> FSGSEATAAILSRAPWSLQSVNPGLKTNSSKEPKFTKCRSPERETFSCHWTDEVHHGTKNLGPIQLFYTRRNTQEWTQEWKECPDYVSAGENSCYFNSSFTSIWIPYCIKLTSNGGTVDEKCFSVDEIVQPDPPIALNWTLLNVSLTGIHADIQVRWEAPRNADIQKGWMV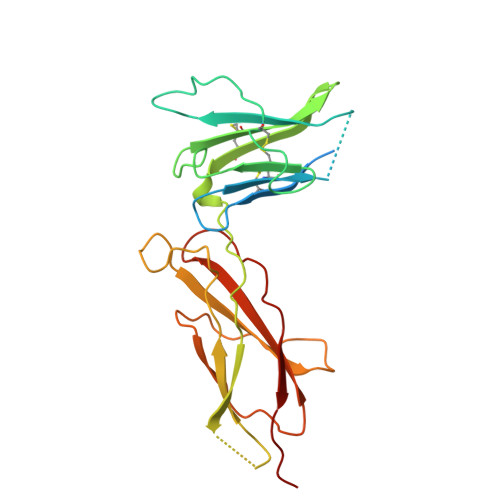LEYELQYKEVNETKWKMMDPILTTSVPVYSLKVDKEYEVRVRSKQRNSGNYGEFSEVLYVTLPQMSQ The protein product of the Casitas B-lineage lymphoma (c-Cbl) gene is a multi-domain, multi-functional scaffolding protein with E3-ubiquitin ligase activity that is crucial for regulating cell signaling pathways. c-Cbl regulates cell proliferation, differentiation and morphology in response to growth factors, hormones and cytokines, binding to substrates via its tyrosine-kinase binding motif (TKB) in its N-terminus. The c-Cbl TKB domain consists of three tightly-connected domains: a divergent SH2 domain that binds to the phosphorylated tyrosine; a four-helix bundle (4H) which packs against the SH2 domain and completes the phosphotyrosine binding pocket; and a calcium-binding EF-hand, which wedges between the SH2 and 4H domains. Consistent with other studies, our previous study demonstrated that the pSpry2 and pEGFR peptides interact with c-Cbl TKB through (1) a positively-charged pocket into which the phosphorylated tyrosine inserts and establishes the majority of the hydrogen bonds, and (2) a hydrophobic cluster, which forms significant interactions with the conserved C-terminal proline residue of the bound peptide. We also determined the crystal structure of the doubly phosphorylated EGFR and Spry2 peptides complexed with c-Cbl TKB at 2.2 and 2.1 Å resolutions, respectively, and observed that the phosphate group of the Ser/Thr residue shifts away from the c-Cbl phosphotyrosine binding pocket with minor conformational changes of the peptides in the interacting region.

While there is an abundance of evidence both in vitro and in vivo to show that phosphorylation of Tyr1069 on EGFR is crucial for c-Cbl binding and receptor ubiquitination, it is less-well characterized how phosphorylation of the additional serine residues within the target sequence affects substrate recognition by c-Cbl. Recent work has revealed that both Ser1070 and Ser1071, immediately adjacent to the Tyr1069 are critical for EGFR desensitization, internalization and degradation. Similarly, the additional phosphorylation on EGFR significantly reduced the binding affinity of EGFR to Cbl when compared with the singly phosphorylated EGFR peptide, with 26- and 31-fold decreases for ppEGFR and tpEGFR, respectively. Notably, the difference between the double and triple phosphorylation for EGFR was not considerable, suggesting that phosphorylation at the pY+1 position is predominantly responsible for the decrease in binding affinity. Surprisingly, unlike the phosphate group of the tyrosine residue, which makes six hydrogen bonding contacts with c-Cbl, the phosphate groups of Thr56 and Ser1070 have no interaction with c-Cbl and are both shifted away from the surface. When we analyzed the electrostatic surface potential, the results showed that the region on c-Cbl contacting the pY+1 and pY+2 positions of the peptides is negatively charged, which could repel the high negative charge on the phosphorylated serine or threonine residues.

> DSFLQRYSSDPT;> GSLIGLMKDAFQPHHHHHHHLSPHPPGTVDKKMVEKCWKLMDKVVRLCQNPKLALKNSPPYILDLLPDTYQHLRTILSRYEGKMETLGENEYFRVFMENLMKKTKQTISLFKEGKERMYEENSQPRRNLTKLSLIFSHMLAELKGIFPSGLFQGDTFRITKADAAEFWRKAFGEKTIVPWKSFRQALHEVHPISSGLEAMALKSTIDLTCNDYISVFEFDIFTRLFQPWSSLLRNWNSLAVTHPGYMAFLTYDEVKARLQKFIHKPGSYIFRLSCTRLGQWAIGYVTADGNILQTIPHNKPLFQALIDGFREGFYLFPDGRNQNPDLTG[1-(4-chlorophenyl)-1,2,3-triazol-4-yl]methanol 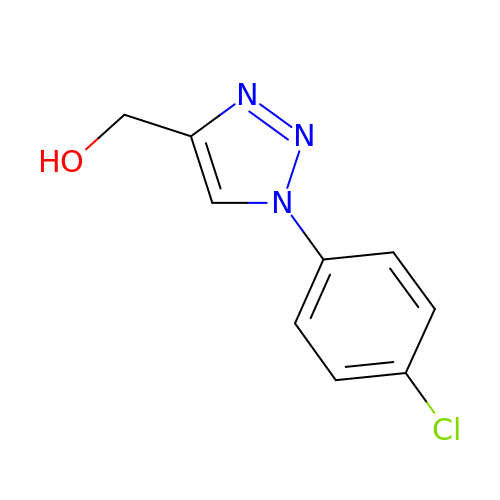| C9 H8 Cl N3 O | CAHIFLPAMJOAGI-UHFFFAOYSA-N> ATVKQPSIGRYTGKPNPSTGKYTVSFIEGDGIGPEISKSVKKIFSAANVPIEWESCDVSPIFVNGLTTIPDPAVQSITKNLVALKGPLATPIGKGHRSLNLTLRKTFGLFANVRPAKSIEGFKTTYENVDLVLIRENTEGEYSGIEHIVCPGVVQSIKLITRDASERVIRYAFEYARAIGRPRVIVVHKSTIQRLADGLFVNVAKELSKEYPDLTLETELIDNSVLKVVTNPSAYTDAVSVCPNLYGDI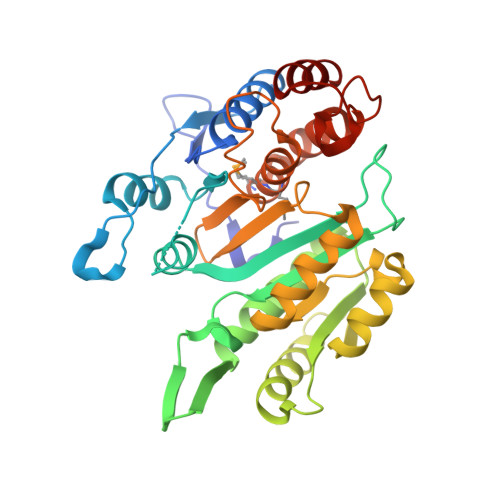LSDLNSGLSAGSLGLTPSANIGHKISIFEAVHGSAPDIAGQDKANPTALLLSSVMMLNHMGLTNHADQIQNAVLSTIASGPENRTGDLAGTATTSSFTEAVIKRL> QETLVRPKPLLLKLLKSVGAQKDTYTMKEVLFYLGQYIMTKRLYDEKQQHIVYCSNDLLGDLFGVPSFSVKEHR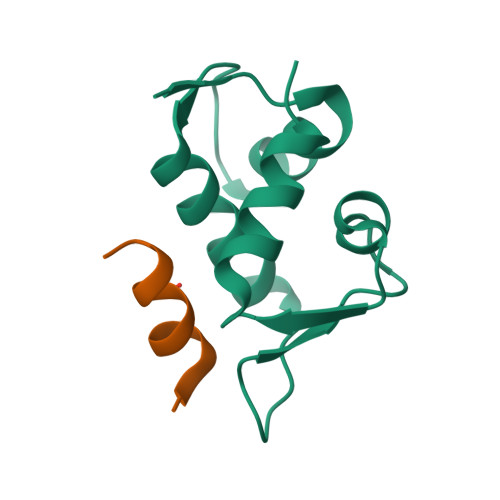KIYTMIYRNLVV;> ETFEHWWSQLLS> PAMTSSDLPLNFQGSPCSQIWQHPRFAAKKRSSMVKFHCYTNHSGALTWFRKRGSQQPQELVSEEGRIVQTQNGSVYTLTIQNIQYEDNGIYFCKQKCDSANHNVTDSCGTELL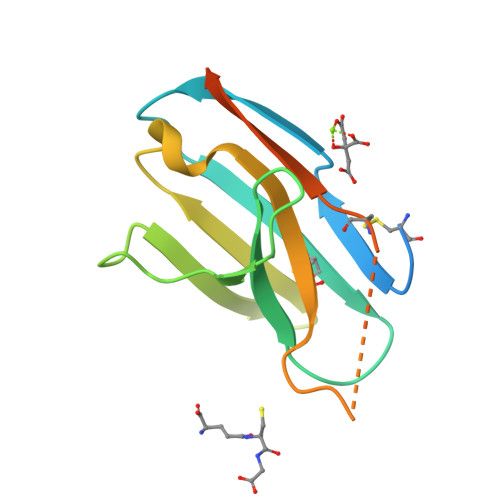VLGFSTLDQLKRRNTLKDG> GLPTMNTPGSTQFLTSDDFQSPCALPQFDVTPSMNIPGEVKNLMEIAEVDSVVPVNNVQDTTDQMEMFRIPVTINAPLQQQVFGLRLQPGLDSVFKHTLLGEILNYYAHWSGSMKLTFVFCGSAMATGKFLIAYSPPGANPPKTRKDAMLGTHIIWDIGLQSSCVLCVPWISQTHYRLVQQDEYTSAGYVTCWYQTGMIVPPG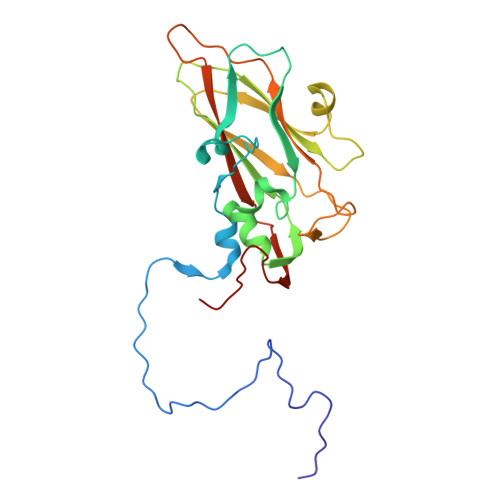TPNSSSIMCFASACNDFSVRMLRDTPFISQDNKLQ>MTDLKASSLRALKLMDLTTLKDDDTDEKVIALCHQAKTPVGNTAAICIYPRFIPIARKTLKEQGTPEIRIATVTNFPHGNDDIDIALAETRAAIAYGADEVDVVFPYRALMAGNEQVGFDLVKACKEACAAANVLLKVIIETGELKDEALIRKASEISIKAGADFIKTSTGKVAVNATPESARIMMEVIRDMGVEKTVGFKPAGGVRTAEDAQKYLAIADELFGADWADA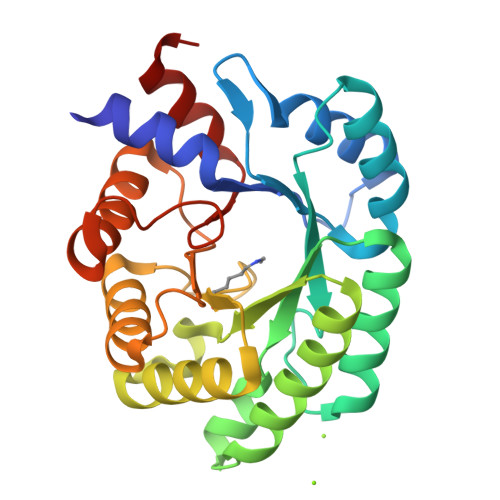RHYRFGASSLLASLLKALGH[2x]> KNNTLWTGPKPEANCIIEYGKQNPDSKLTLILVKNGGIVNGYVTLMGASDYVNTLFKNKNVSINVELYFDATGHILPDSSSLKTDLELKYKQTADFSARGFMPSTTAYPFVLPNAGTHNENYIFGQCYYKASDGALFPLEVTVMLNKRLPDSRTSYVMTFLWSLNAGLAPETTQATLITSPFTFSYIREDD;> VLDINDNEPVFTQDVFVGSVEELSAAHTLVMKINATDADEPNTLNSKISYRIVSLEPAYPPVFYLNKDTGEIYTTSVTLDREEHSSYTLTVEARDGNGEVTDKPVKQAQVQIRILDVNDNIPVVENKVLEGMVEENQVNVEVTRIKVFDADEIGSDNWLANFTFASGNEGGYFHIETDAQTNEGIVTLIKEVDYEEMKN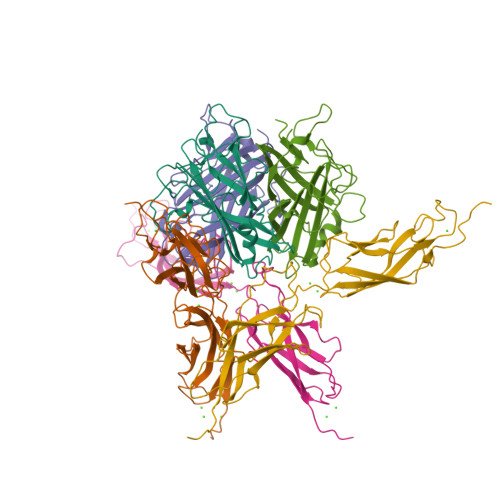LDFSVIVANKAAFHKSIRSKYKPTPIPIKVKVKNVKEGI>[4x]MTRQVLVTGASKGIGKAIAVQLAKDGFHIVVHYMGDQQGAQNTLETIEQHGGSGRLIQFDISNREECRTKLEADIAEHGAYYGVVNNAGITRDTAFPAMTEEEWDGVIHTNLD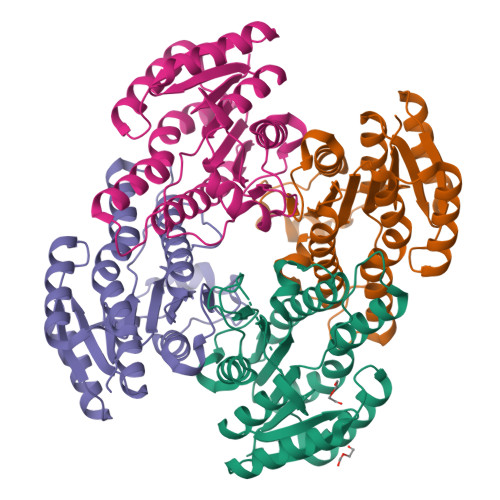SFYNVLHPCVMPMVQKRKGGRIVTLASVSGLMGNRGQTNYSAAKAGVIGATKSLALELAKRKITVNCVAPGLIDTGMVDEHVKEHAMPQIPLRRMGEPEEVAGLVSYLMSDIAGYVTRQVISVNGGLV> D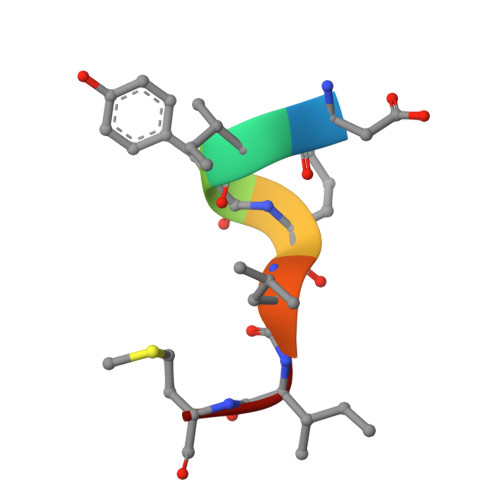IYQLIM>[4x]MHHHHHHSTPSIVIASAARTAVGSFNGAFANTPAHELGATVISAVLERAGVAAGEVNEVILGQVLPAGEGQNPARQAAMKAGVPQEATAWGMNQLCGSGLRAVALGMQQIATGDASIIVAGGMESMSMAPHCAHLRGGVKMGDFKMIDTMIKDGLTDAFYGYHMGTTAENVA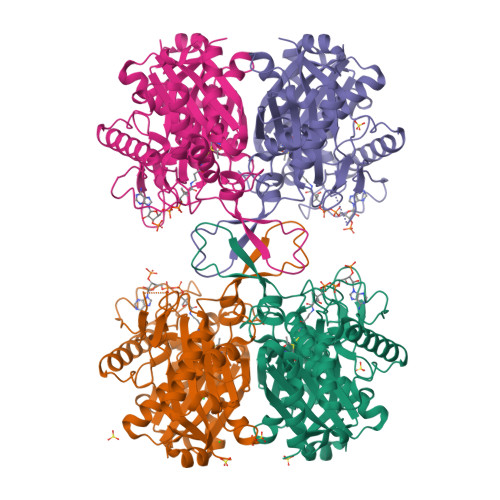KQWQLSRDEQDAFAVASQNKAEAAQKDGRFKDEIVPFIVKGRKGDITVDADEEIRGATLDSMAKLRPAFDKEGTVTAGNASGLNDGAAAALLMSEAEASRRGIQPLGRIVSWATVGVDPKVMGTGPIPASRKALERAGWKIGDLDLVEANEAFAAQACAVNKDLGWDPSIVNVNGGAIAIGHPIGASGARILNTLLFEMKRRGARKGLATLCIGGGMGVAMCIESL> EPIRYAIPEELDRGSLVGNLAKDLGFGVGDLPTRNLRVIAEKKFFTVSPENGNLLVSDRIDREEICGKKSTCVLEFEMVAEKPLNFFHVTVLIQDINDNPPTFSQNITELEISELALTGATFALESAQDPDVGVNSLQQYYLSPDPHFSLIQKENLDGSRYPELVLKAPLDREEQPHHHLVLTAVDGGEPSRSCTTQIRVIVADANDNPPVFTQDMYRVNVAENLPAGSSVLKVMAIDMDEGINAEIIYAFINIGKEVRQLFKLDSKTGELTTIGELDFEERDSYTIGVEAKDGGHHTAYCKVQIDISDENDNAPEITLASESQHIQEDAELGTAVALIKTHDLDSGFNGEILCQLKGNFPFKIVQDTKNTYRLVTDGALDREQIPEYNVTITATDKGNPPLSSSKTITLHILD

Protocadherins (Pcdhs) encompass about 70% of the cadherin superfamily in mammals, and are involved in cell adhesion in the nervous system of higher animals. Clustered Pcdhs, comprising the α, β, and γ subfamilies, mediate neuronal survival, self-avoidance and self/nonself discrimination, and promote dendritic arborization in neuronal cells. For example, Pcdh7 is involved in germ layer differentiation, and Pcdh1 and Pcdh8 mediate cell sorting and migration during gastrulation. Both clustered and non-clustered Pcdhs control these phenotypes through homophilic interactions of their extracellular cadherin (EC) repeat domains. Using sequence co-evolution analysis, we predicted intersubunit EC1-EC4 interactions, and proposed that clustered Pcdhs form extended antiparallel homodimers engaging EC1-4.

We determined the crystal structure of PcdhγB3 EC1-4, the first full antiparallel dimer for a γ isoform. Based on multi-angle light scattering (MALS), peak 1 was wide and polydisperse (~200–300 kDa). Peak 2 was monodisperse at 80 kDa – consistent with a dimer – and readily yielded a crystal structure (Figure 1—source data 1). Although the asymmetric unit contains a single PcdhγB3 molecule, a crystallographic two-fold axis generates an antiparallel dimer with intersubunit EC1/EC4 and EC2/EC3 interactions. This dimer is consistent with the PcdhγA1 EC1-3 crystal structure, validating the previously predicted interface, and with recent α and β Pcdhs structures, confirming that this interaction mechanism is conserved among all clustered Pcdh subfamilies. As expected, each EC forms a seven-stranded Greek key β-sandwich motif, similarly to other clustered Pcdh structures. Notably, EC4 has a unique β-strand arrangement compared to EC1-EC3 and all known cadherin repeat structures. Third, the PcdhγB3 EC1/EC4 interface is much larger (BSA = 976 Å2 per protomer) than the EC2/EC3 interface (555 Å2 per protomer). In the PcdhγB3 EC1/EC4 interface, F86, one of the predicted affinity-driving residues from EC1, wedges into a cavity created by hydrophobic EC4 residues. A PcdhγB3 EC1-4 F86A mutant indeed disrupted dimerization, resulting in a monomeric protein as measured by MALS. Analogously, purified EC1-3 constructs failed to dimerize in vitro whereas EC1-4 constructs did, and K562 cells expressing ΔEC1 or ΔEC4-6 constructs did not aggregate while cells expressing chimeras in which EC1 and EC4 derived from different paralogs did. Together, these results indicate that the EC1/EC4 interaction is not strictly required for the specificity of dimerization but it drives dimerization affinity through non-specific hydrophobic interactions.>[2x]MRGSHHHHHHGSVTCTGCVDLDELSFEKTVERFPYSVVKFDIAYPKGEKHEAFTAFSKSAHK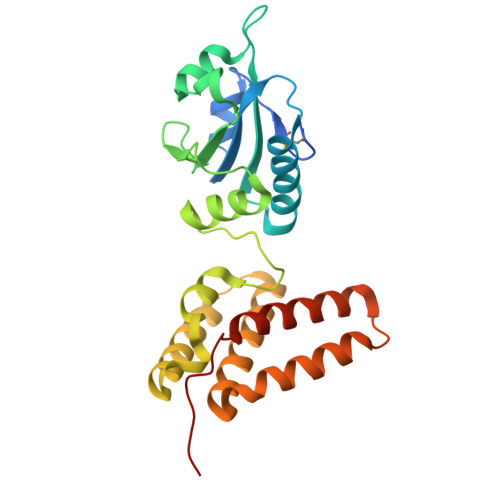ATKDLLIATVGVKDYGELENKALGDRYKVDDKNFPSIFLFKGNADEYVQLPSHVDVTLDNLKAFVSANTPLYIGRDGCIKEFNEVLKNYANIPDAEQLKLIEKLQAKQEQLTDPEQQQNARAYLIYMRKIHEVGYDFLEEETKRLLRLKAGKVTEAKKEELLRKLNILEVFRVHKVTKTAPEKEEL> MENTENSVDSKSIKNLEPKIIHGSESMDSGISLDNSYKMDYPEMGLCIIINNKNFHKSTGMTSRSGTDVDAANLRETFRNLKYEVRNKNDLTREEIVELMRDVSKEDHSKRSSFVCVLLSHGEEGIIFGTNGPVDLKKITNFFRGDRCRSLTGKPKLFIIQACRGTELDCGIETDSGVDDDMACHKIPVEADFLYAYSTAPGYYSWRNSKDGSWFIQSLCAMLKQYADKLEFMHILTRVNRKVATEFESFSFDATFHAKKQI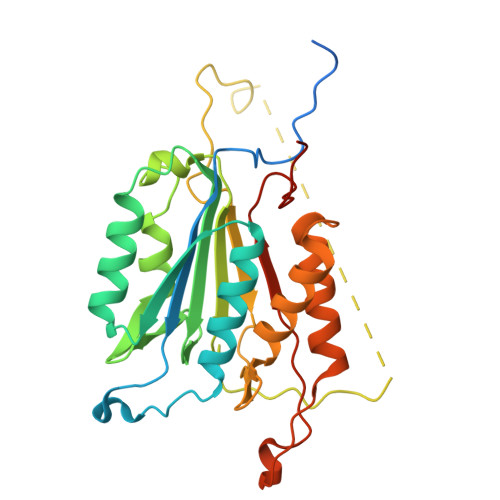PCIVSMLTKELYFYHQLHHHHHH>[2x]MTSIFHFAIIFMLILQIRIQLSEESEFLVDRSKNGLIHVPKDLSQKTTILNISQNYISELWTSDILSLSKLRILIISHNRIQYLDISVFKFNQELEYLDLSHN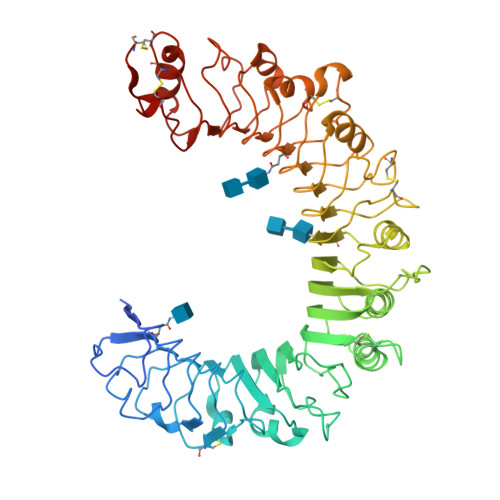KLVKISCHPTVNLKHLDLSFNAFDALPICKEFGNMSQLKFLGLSTTHLEKSSVLPIAHLNISKVLLVLGETYGEKEDPEGLQDFNTESLHIVFPTNKEFHFILDVSVKTVANLELSNIKCVLEDNKCSYFLSILAKLQTNPKLSNLTLNNIETTWNSFIRILQLVWHTTVWYFSISNVKLQGQLDFRDFDYSGTSLKALSIHQVVSDVFGFPQSYIYEIFSNMNIKNFTVSGTRMVHMLCPSKISPFLHLDFSNNLLTDTVFENCGHLTELETLILQMNQLKELSKIAEMTTQMKSLQQLDISQNSVSYDEKKGDCSWTKSLLSLNMSSNILTDTIFRCLPPRIKVLDLHSNKIKSIPKQVVKLEALQELNVASNQLKSVPDGIFDRLTSLQKIWLHTNPWDCSCPRIDYLSRWLNKNSQKEQGSAKCSGSGKPVRSIICPT>MKRFFNRFYLDTGIIADPSQRSLASRVSAFLVQGAVAFSLLGTIGVDTSPLIAAAGVTGATIGFACKDFGTNFVASIVLSGQQSIRTGNLVCIGTGLNVVKGKVVDWDTRYLYLRSSEGHLLHVPNNMVLNSVVTWEQEKKQNPHETDLPKQDVVKAPGDNAAKQSNSLEVLFQ[7x]

Trypanosoma cruzi, the protozoan parasite causing Chagas disease, encodes a miniature MscS ortholog (TcMscS) critical for parasite development and infectivity. TcMscS contains a minimal portion of the canonical EcMscS fold yet maintains mechanosensitive channel activity, thus presenting a unique model system to assess the essential molecular determinants underlying mechanotransduction. By combining electrophysiology, single-particle cryo-EM, and all-atom molecular dynamics (MD) simulations, we show that TcMscS forms a heptameric channel with a central ion conduction path, but indeed lacks the side portals shared by other MscS-like channels. Strikingly, the presumed two TM helices are of insufficient length to fully cross an intact planar lipid membrane and thus induce drastic membrane deformation surrounding the channel.

The full-length TcMscS, consisting of 165 amino acids, was heterologously expressed in Pichia pastoris, purified to homogeneity in glyco-diosgenin (GDN) detergents, and subjected to single-particle cryo-EM analysis. The 3D reconstruction reached an overall resolution of 3.21 Å with applied C7 symmetry. The C-terminal region, including amino acids 138–165, was not resolved in the cryo-EM density map and thus not included in the atomic model. Alignment of the conserved β domains in these structures indicates that the arrangement of TM2 and TM3 in TcMscS is similar to that in the open EcMscS channel but differs substantially from that in the closed, suggesting that the TcMscS structure may represent an open conformation and that TcMscS adopts a membrane-embedded position closer to that of the open EcMscS channel. Comparison of the pore profiles of TcMscS and closed and open EcMscS channels indicates that the transmembrane region of TcMscS has an intermediate opening, with the narrowest pore diameter of 10.8 Å at residue F64. The structures of TcMscS in detergents and in nanodiscs are essentially identical, with an RMSD of ~ 0.3 Å for all Cα atoms. Thus, this conformation is inherently favored by the purified wild-type TcMscS channel, either in detergent or lipid environment. However, a wealth of lipid-like densities is associated with the channel, evident in the cryo-EM density map of TcMscS in detergent or in lipid, which may interfere with ion conduction. Estimation of the pore radius with the inclusion of lipids in the atomic model rendered a hydrophobic region with much reduced opening, comparable to that of the closed EcMscS channel. Therefore, it appears that the resident pore lipids occlude ion conduction, and that channel activation would require departure of the pore lipids from the central ion permeation path.>AGFQLNEFSSSGLGRAYSGEGAIADDAGNVSRGGGLITMFDRPTFSAGAVYIDPDVNISGTSPSGRSLKADNIAPTAWVPNMHFVAPINDQFGWGASITSNYGLATEFNDTYAGGSVGGTTDLETMNLNLSGAYRLNNAWSFGLGFNAVYARAKIERFAGDLGQLVAGQIMQSPAGQTQQ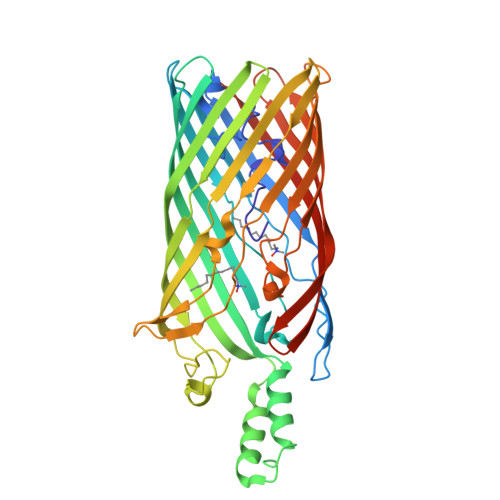GQALAATANGIDSNTKTAHLNGNQWGFGWNAGILYELDKNNRYALTYRSEVKIDFKGNYSSDLNRAFNNYGLPIPTATGGATQSGYLTLNLPEMWEVSGYNRVDPQWAIHYSLAYTSWSQFQQLKATSTSGDTLFQKHEGFKDAYRIALGTTYYYDDNWTFRTGIAFDDSPVPAQNRSISIPDQDRFWLSAGTTYAFNKDASVDVGVSYMHGQSVKINEGPYQFESEGKAWLFGTNFNYAFHHHHHH[2x]> MMFGRFTERAQKVLALAQEEALRLGHNNIGTEHILLGLVREGEGIAAKALQALGLGSEKIQKEVESLIGRGQEMSQTIHYTPRAKKVIELSMDEARKLGHSYVGTEHILLGLIREGEGVAARVLNNLGVSLNKARQQVLQLLGSNETGSSAAGTNSNANTPTLDSLARDLTAIAKEDSLDPVIGRSKEIQRVIEVLSRRTKNNPVLIGEPGVGKTAIAEGLAQQIINNEVPEILRDKRVMTLDMGTVVAGTKYRGEFEDRLKKVMDEIRQAGNIILFIDALHTLIGAGGAEGAIDASNILKPSLARGELQCIGATTLDEYRKYIEKDAALERRFQPIQVDQPSVDESIQILQGLRDRYEAHHRVSITDDAIEAAVKLSDRYISDRFLPDKAIDLIDEAGSKVRLRSFTTPPNLKELEQKLDEVRKEKDAAVQSQEFEKAASLRDTEQRLREQVEDTKKSWKEKQGQENSEVTVDDIAMVVSSWTGVPVSKIAQTETDKLLNMENILHSRVIGQDEAVVAVAKAVRRARAGLKDPKRPIGSFIFLGPTGVGKTELARALAESIFGDEESMIRIDM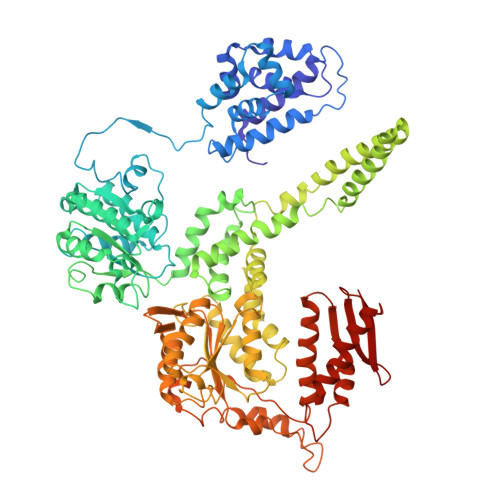SEYMEKHSTSRLVGSPPGYVGYDEGGQLTEKVRRKPYSVVLLDEIEKAHPDVFNILLQVLEDGRLTDSKGRTVDFRNTILIMTSNVGASELKRNKYVGFNVQDETQNHKDMKDKVMGELKRAFRPEFINRIDEIIVFHSLEKKHLTEIVSLMSDQLTKRLKEQDLSIELTDAAKAKVAEEGVDLEYGARPLRRAIQKHVEDRLSEELLRGNIHKGQHIVLDVEDGEFVVKTTAKTN>MALLAEHLLKPLPADKQIETGPFLEAVSHLPPFFDCLGSPVFTPIKADISGNITKIKAVYDTNPAKFRTLQNILEVEKEMYGAEWPKVGATLALMWLKRGLRFIQVFLQSICDGERDENHPNLIRVNATKAYEMALKKYHGWIVQKIFQAALYAAPYKSDFLKALSKGQNVTEEECLEKIRLFLVNYTATIDVIYEMYTQMNAELNYKV[4x]

Human glycolipid transfer protein (hsGLTP) forms the prototypical GLTP fold and is characterized by a broad transfer selectivity for glycosphingolipids (GSLs). In human GLTP, a glycolipid headgroup recognition centre located on the protein surface enables selective binding of the GSL head and ceramide amide groups via multiple specific interactions. Encapsulation of lipid chains within the hydrophobic pocket involves a cleft-like gating mechanism that results in two glycolipid-binding modes. To elucidate the structural dynamics of the GLTP–GSL dimer and associated adaptations, we comparatively analyzed nine novel crystal structures of wild-type GLTP (wtGLTP) and the sulfatide-specific mutants D48V and A47D/D48V complexed with N-lauroyl-containing monosulfatide (N-lauroyl-3-O-sulfo-galactosylceramide; hereafter referred to as 12:0 monoSF) and disulfatide (N-lauroyl-3,6-di-O-sulfo-galactosylceramide; hereafter referred to as 12:0 diSF) in different crystal forms and compared them with previously studied GLTP–24:1 monoSF complexes.

Although the crystal packing differs in various crystal forms, we found a similar dimeric structure in all crystals, indicating the non-randomness of GLTP–SF homodimerization. In crystal form 3, the four molecules comprising the asymmetric unit form two dimers similar to the original C2 dimer. To further assess the intrinsic nature of these variations, two dimers belonging to the same crystal were analyzed for changes in dimer openness. The observed differences are comparable with those found in different complex types belonging to isomorphous crystals. Even within the same complex, 12:0-monoSF–wtGLTP, the θ angle and t distance vary significantly in the different crystal forms (68.2–80.2° and 15.4–19.5 Å, respectively), reflecting changes in dimer openness. In class 2 crystals, N is 2, 4 or 1, indicating the potential structural distinctions between monomers which are not related by crystallographic symmetry.>GSHMVERISLEKAALEFSEANAPHPRIYELPVEEGRSLLNEVQDSPVVKEDVDIEDIAVDTGEWGEINVRFIRPLHQEKKLPVIFYIHGAGWVFGNAHTHDKLIRELAVRTNSVVVFSEYSLSPEAKYPTAIEQNYAVLQQLKDFANDKKFDVNHLTVAGD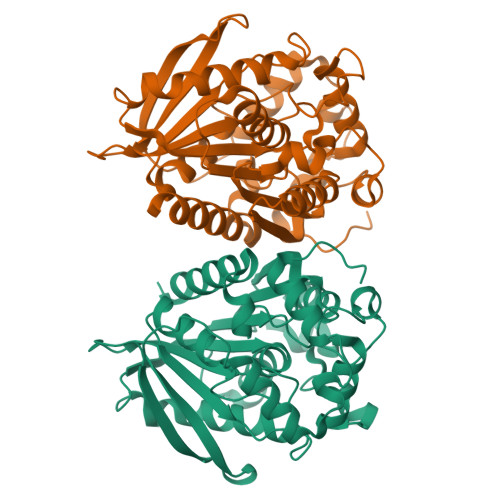SVGGNMATVMTLLTKQRGGQKIGQQVLYYPVTDANFDTDSYNEFAENYALTKEGMIWFWDQYTTSQEERHQITASPLRATKEDLADLPAALIITGEADVLRDEGEAYARKLREADVEVTQVRFQAIIHDFVMVNSMNETHATRAAMSLSTQWINEKNRK[8x]1,3-dimethyl-8-{[2-(morpholin-4-yl)ethyl]sulfanyl}-3,7-dihydro-1H-purine-2,6-dione 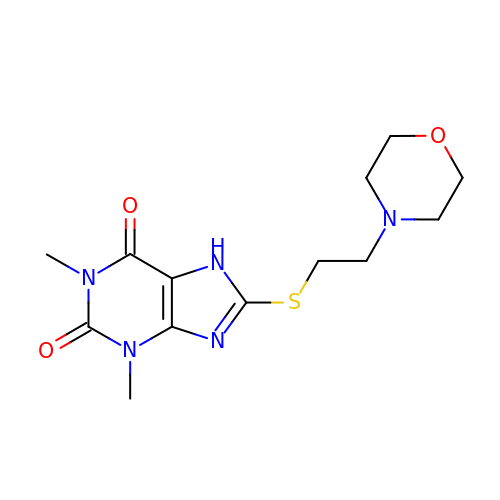| C13 H19 N5 O3 S | ZLIJABXMFRYUIA-UHFFFAOYSA-N> KSAQQELKQRQRAE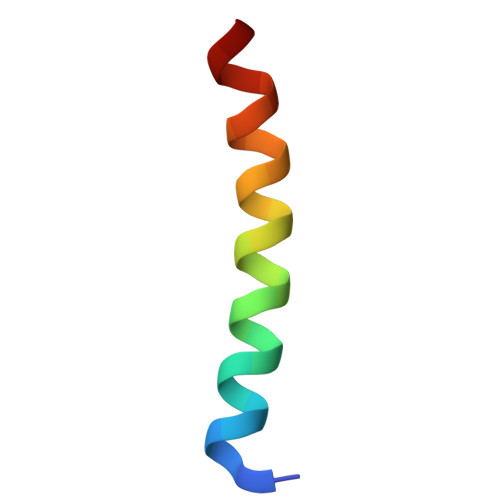IYALNRVMTELEQQ>[2x]GSHMVRESSFVEKMKKTGRNIIVFYGSQTGTAEEFANRLSKDAHRYGMRGMSADPEEYDLADLSSLPEIDNALVVFCMATYGEGDPTDNAQDFYDWLQETDVDLSGVKFAVFGLGNKTYEHFNAMGKYVDKRLEQLGAQRIFELGLGDDDGNLEEDFITWREQFWPAVCEHFGVEATGEESSIRQYELVVHTDIDAAKVYMGEMGRLKSYENQKPPFDAKNPFLAAVTTNRKLNQGTERHLMHLELDISDSKIRYESGDHVAVYP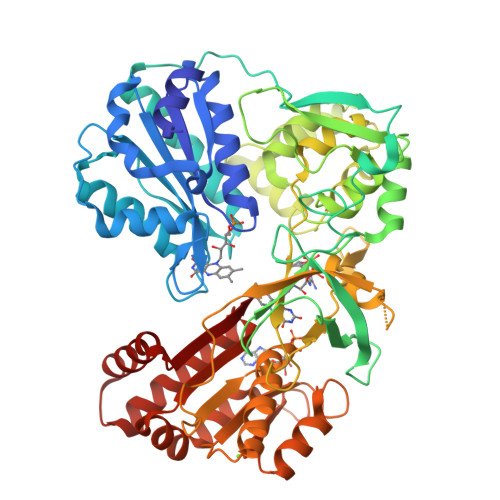ANDSALVNQLGKILGADLDVVMSLNNLDEESNKKHPFPCPTSYRTALTYYLDITNPPRTNVLYELAQYASEPSEQELLRKMASSSGEGKELYLSWVVEARRHILAILQDCPSLRPPIDHLCELLPRLQAHYYSIASSSKVHPNSVHICAVVVEYETKAGRINKGVATNWLRAKEPAGENGGRALVPMFVRKSQFRLPFKATTPVIMVGPGTGVAPFIGFIQERAWLRQQGKEVGETLLYYGCRRSDEDYLYREELAQFHRDGALTQLNVAFSREQSHKVYVQHLLKQDREHLWKLIEGGAHIYVCGDARNMARDVQNTFYDIVAELGAMEHAQAVDYIKKLMTKGRYSLDVWS> MRDADADAGGGADGGDGRGGHSCRGGVDTAAAPAGGAPPAHAPGPGRDAASAARGSRMRPHIFTLSVPFPTPLEAEIAHGSLAPDAEPHQRVVGKDLTVSGRILVVRWKAEDCRLLRISVINFLDQLSLVVRTMQRFGPPVSR;> MELLGEYVGQEGKPQKLRVSCEAPGDGDPFQGLLSGVAQMKDMVTELFDPLVQGEVQHRVAAAPDEDLDGDDEDDAEDENNIDNRTNFDGPSAKRPKTPSHHHHHH;> MPAVLGFEGSANKIGVGVVRDGKVLANPRRTYVTPPGTGFLPGDTARHHRAVILDLLQEALTESGLTSQDIDCIAYTKGP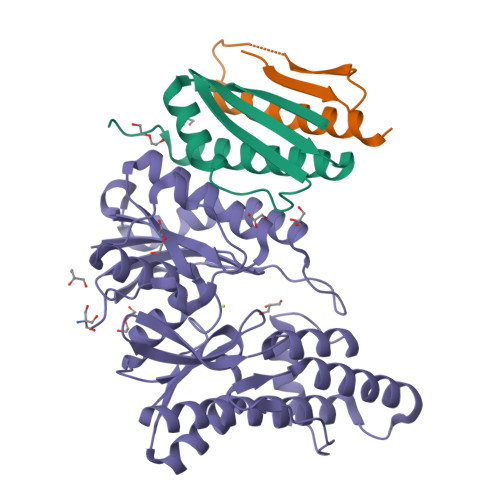GMGAPLVSVAVVARTVAQLWNKPLVGVNHCIGHIEMGRLITGATSPTVLYVSGGNTQVIAYSEHRYRIFGETIDIAVGNCLDRFARVLKISNDPSPGYNIEQMAKRGKKLVELPYTVKGMDVSFSGILSFIEDVAHRMLATGECTPEDLCFSLQETVFAMLVEITERAMAHCGSQEALIVGGVGCNVRLQEMMATMCQERGARLFATDERFCIDNGAMIAQAGWEMFRAGHRTPLSDSGVTQRYRTDEVEVTWRD> MHDPIPTIAFPDGRKVPALGQGTWRMGENRAKTADEVRSLQTGLDLGMTLIDTAEMYGDGAAERIVGEAIKGRRDEAFVVSKVLPSNASRAGTVAACERSLRNLGIDCVDLYLLHWRGGYPLAETVAAFEELKKAGKIRAWGVSNFDVDDMEELSAVPDGGNVAANQVLYNLARRGIEFDLLPRCRAQGVPVMAYSPLDEGRLLHDADLIHIAKAHQATPAQVALAFLKTCSGVISIPKTGS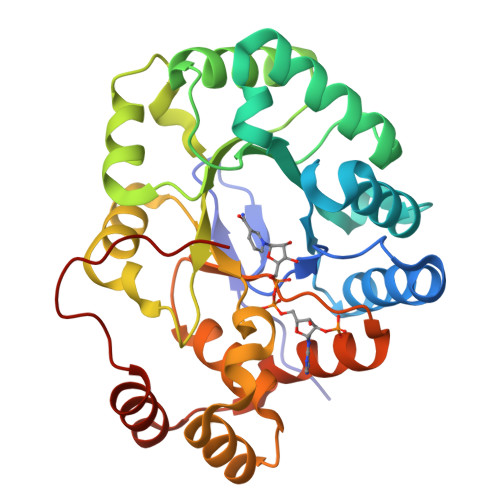PERARENRDAMDIHLTTENLAELDRHFPPPRRKTRLEVI>[2x]AQPAARDLKVVTKRGSADGCTDWSVDIKKYQVLVGEPVRIKCALFYGYIRTNYSLAQSAGLSLMWYKSSGPGDFEEPIAFDGSRMSKEEDSIWFRPTLLQDSGLYACVIRNSTYCMKVSISLTVGENDTGLCYNSKMKYFEKAELSKSKEISCRDIEDFLLPTREPEILWYKECRTKAWRPSIVFKRDTLLIKEVKEDDIGNYTCELKYGGFVVRRTTELTVTAPLTDKPPKLLYPMESKLTVQETQLGGSANLTCRAFFGYSGDVSPLIYWMKGEKFIEDLDENRVWESDIRILKEHLGEQEVSISLIVDSVEEGDLGNYSCYVENGNGRRHASVLLHKRKHHHHHH

Vertebrate type-IIa RPTPs comprise LAR, PTPσ and PTPδ, which share common domain architecture with a single transmembrane (TM) helix flanked by a large extracellular domain (ECD) and cytoplasmic tandem PTP domains: the membrane-proximal PTP domain (D1) is catalytically active, whereas the membrane-distal PTP domain (D2) is inactive. In mammals, presynaptic type-IIa RPTPs form trans-synaptic adhesion by specifically binding to their cognate postsynaptic organizers through their ECDs for inducing synaptic differentiation of neurons. To date, five different types of postsynaptic organizers for type-IIa RPTPs have been reported: interleukin-1 receptor (IL-1R) accessory protein (IL-1RAcP)7, IL-1RAcP-like-1 (IL1RAPL1)8, neurotrophin receptor tyrosine kinase C (TrkC), netrin-G ligand-3 (NGL-3)1011 and Slit- and Trk-like (Slitrk) family proteins. To elucidate the structural basis for decoding the ‘splice-insert signaling code' in the type-IIa RPTPs, we determined the crystal structures of PTPδ-ECD in complex with IL-1RAcP-ECD and IL1RAPL1-ECD.

IL1RAPL1-ECD consists of three Ig domains, which are arranged in an L-shape.>[2x]NAQFLHTQVGRGLLGAVVNPLGEVTDKFAVTDNSEILYRPVDNAPPLYSERAAIEKPFLTGIKVIDSLLTCGEGQRMGIFASAGCGKTFLMNMLIEHSGADIYVIGLIGEEGREVTETVDYLKNSEKKSRCVLVYATSDYSSVDRCNAAYIATAIAEFFRTEGHKVALFIDS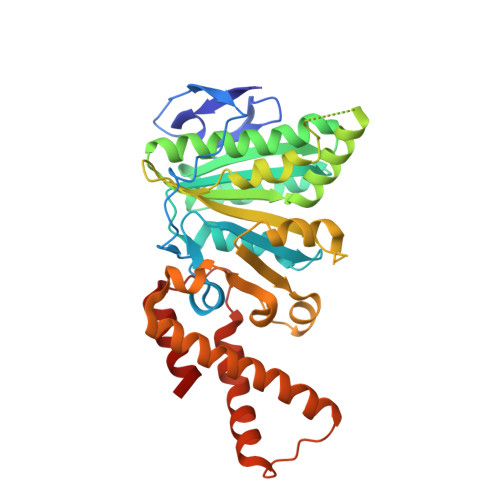LTRYARALRDVALAAGESPARRGYPVSVFDSLPRLLERPGKLKAGGSITAFYTVLLEDDDFADPLAEEVRSILDGHIYLSRNLAQKGQFPAIDSLKSISRVFTQVVDEKHRIMAAAFRELLSEIEELRTIIDFGEYKPGENASQDKIYNKISVVESFLKQDYRLGFTYEQTMELIGETIR> AL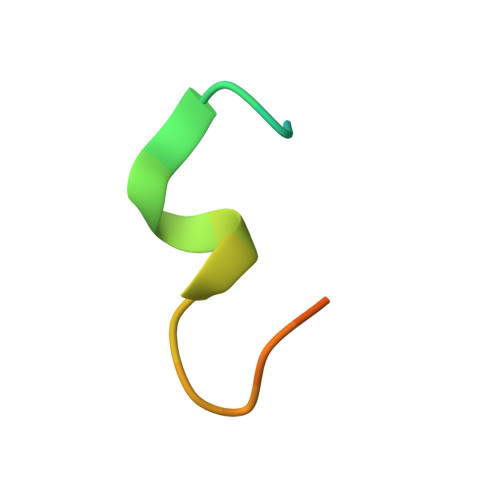NTAKKGLIDYYLMPSLSTTSR>MATQGVFTLPANTRFGVTAFANASGTQTVNVLVNNETAATFSGQSTNNAVIGTQVLNSGSSG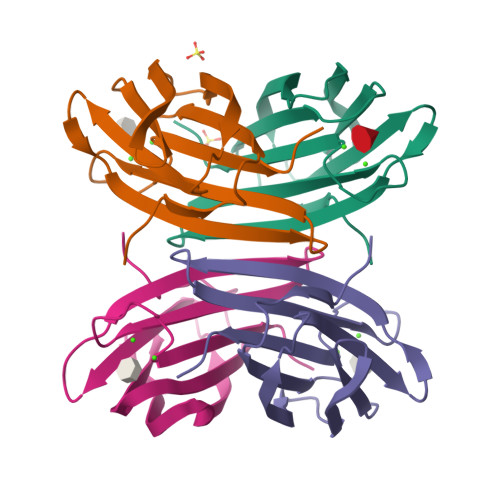KVQVQVSVNGRPSDLVSAQVILTNELNFALVGSEDGTDNDYNDAVVVINWPLG[4x]(1R,3R,7E,17beta)-17-{(1R,2E,4R)-4-hydroxy-1-methyl-4-[(3S,5S,7S)-tricyclo[3.3.1.1~3,7~]dec-1-yl]but-2-en-1-yl}-2-methylidene-9,10-secoestra-5,7-diene-1,3-diol | C34 H50 O3 | 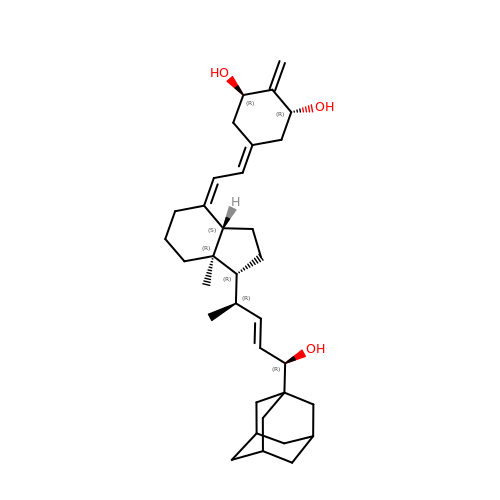XEQPVMGAXBNZAH-XMMQUESESA-N> MAKEWGYASHNGPDHWHELFPNAKGENQSPIELHTKDIRHDPSLQPWSVSYDGGSAKTILNNGKTCRVVFDDTYDRSMLRGGPLPGPYRLRQFHLHWGSSDDHGSEHTVDGVKYAAELHLVHWNPKYNTFKEALKQRDGIAVIGIFLKIGHENGEFQIFLDALDKIKT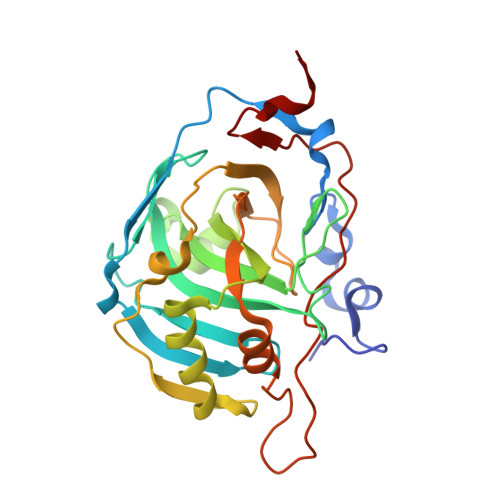KGKEAPFTKFDPSSLFPASRDYWTYQGSFTTPPCEECIVWLLLKEPMTVSSDQMAKLRSLLSSAENEPPVPLVSNWRPPQPINNRVVRASFKHHHHHH1-(6-bromopyridin-3-yl)-1,4-diazepane 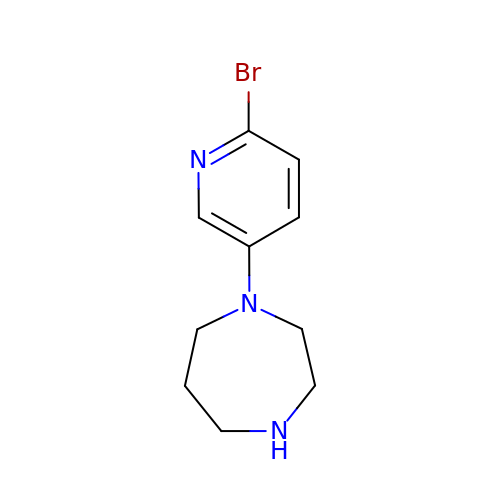| C10 H14 Br N3 | JRNYLCIPPWHNEJ-UHFFFAOYSA-N>[4x]MRVNALLPLSGLIGTALAACPFADPSALGRRAEGGEVDARQRLKEVEVDDNGQFMTTDFGGNIEEQFSLKAGGRGSTLLEDFIFRQKLQHFDHERIPERVVHARGAGAHGIFTSYGDWSNITAASFLGAKDKQTPVFVRFSTVAGSRGSADTARDVHGFATRFYTDEGNFDIVGNNIPVFFIQDAIRFPDLIHSV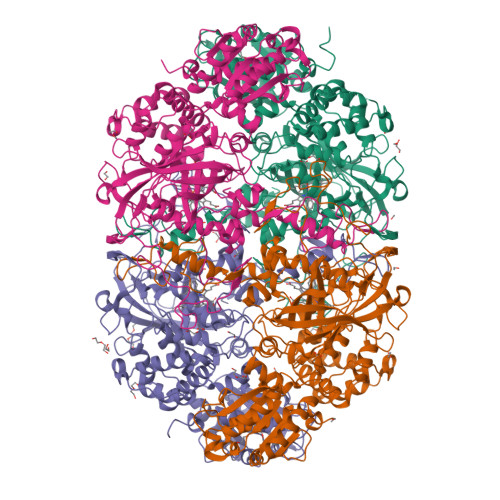KPSPDNEVPQAATAHDSAWDFFSSQPSALHTLFWAMSGNGIPRSYRHMDGFGIHTFRLVTEDGKSKLVKWHWKTKQGKAALVWEEAQVLAGKNADFHRQDLWDAIESGNAPSWELAVQLIDEDKAQAYGFDLLDPTKFLPEEFAPLQVLGEMTLNRNPMNYFAETEQISFQPGHIVRGVDFTEDPLLQGRLYSYLDTQLNRHRGPNFEQLPINRPVSGVHNNHRDGQGQAWIHKNIHHYSPSYLNKGYPAQANQTVGRGFFTTPGRTASGVLNRELSATFDDHYTQPRLFFNSLTPVEQQFVINAIRFEASHVTNEQVKKNVLEQLNKISNDVAKRVAVALGLEAPQPDPTYYHNNVTRGVSIFNESLPTIATLRVGVLSTTKGGSLDKAKALKEQLEKDGLKVTVIAEYLASGVDQTYSAADATAFDAVVVAEGAERVFSGKGAMSPLFPAGRPSQILTDGYRWGKPVAAVGSAKKALQSIGVEEKEAGVYAGAQDEVIKGVEEGLKVFKFLERFAVDGDDEE>[4x]GSVIKQGYLEKKSKDHSFFGSEWQKRWCVV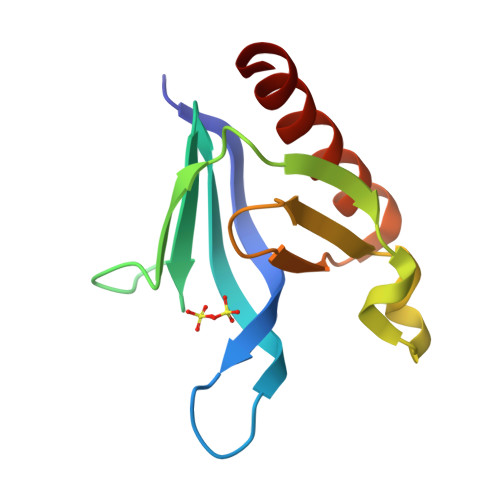SRGLFYYYANEKSKQPKGTFLIKGYSVRMAPHLRRDSKKESCFELTSQDRRTYEFTATSPAEARDWVDQISFLLKDLS> SGDYRVQNTSLEAIVQNASSDNQGIQLSAVQAARKLLSSDRNPPIDDLIKSGILPILVHCLERDDNPSLQFEAAWALTNIASGTSEQTQAVVQSNAVPLFLRLLHSPHQNVCEQAVWALGNIIGDGPQCRDYVISLGVVKPLLSFISPSIPITFLRNVTWVMVNLCRHKDPPPPMETIQEILPALCVLIHHTDVNILVDTVWALSYLTDAGNEQIQMVIDSGIVPHLVPLLSHQEVKVQTAALRAVGNIVTGTDEQTQVVLNCDALSHFPALLTHPKEKINKEAV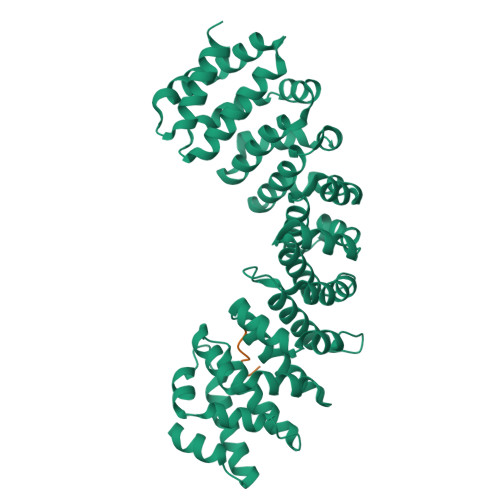WFLSNITAGNQQQVQAVIDANLVPMIIHLLDKGDFGTQKEAAWAISNLTISGRKDQVAYLIQQNVIPPFCNLLTVKDAQVVQVVLDGLSNILKMAEDEAETIGNLIEECGGLEKIEQLQNHENEDIYKLAYEIIDQFFSSDDIDEDPSLVPEAIQGGTFGFNSSANVPTEGFQF;> VQLRRKSDLETSEPKPFLYYPEIKDKEEVQRKRQKLMPNF> A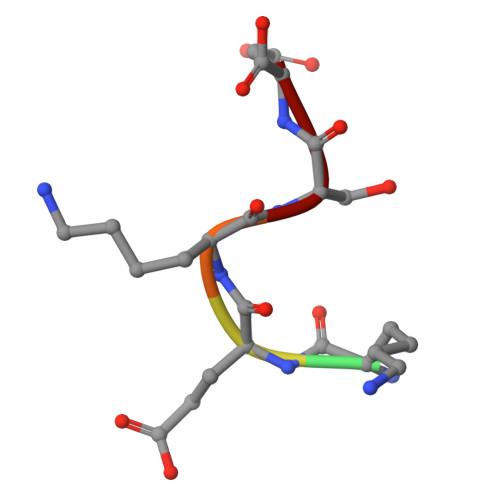KEKSD> QEP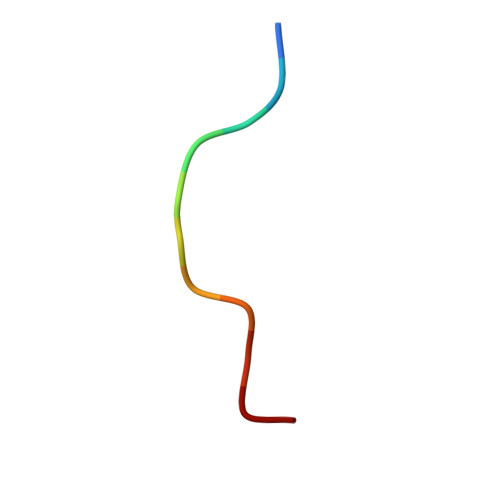EGSGGGQG> MHRTTRIKITELNPHLMCVLCGGYFIDATTII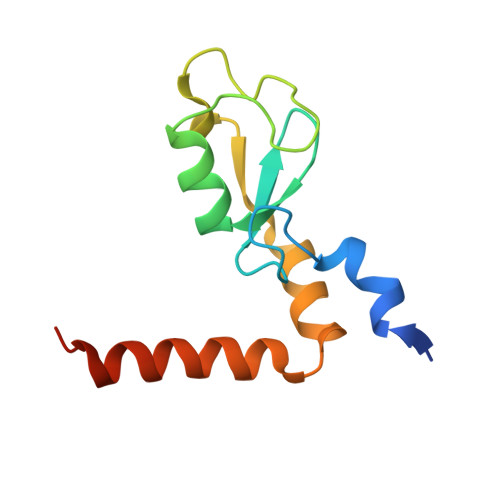ECLHSFCKTCIVRYLETSKYCPICDVQVHKTRPLLNIRSDKTLQDIVYKLVPGLFKNEMKRRRDFYAAHPSADAAN>[8x]GIDPFTNTKWDYKNKENGPHRWDKLHKDFEVC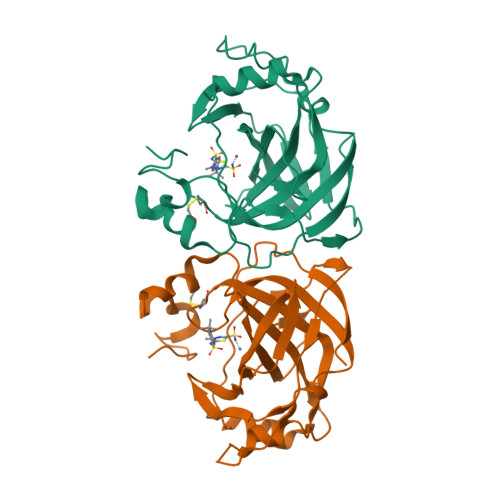KSGKSQSPINIEHYYHTQDKADLQFKYAASKPKAVFFTHHTLKASFEPTNHINYRGHDYVLDNVHFHAPMEFLINNKTRPLSAHFVHKDAKGRLLVLAIGFEEGKENPNLDPILEGIQKKQNFKEVALDAFLPKSINYYHFNGSLTAPPCTEGVAWFVIEEPLEVSAKQLAEIKKRMKNSPNQRPVQPDYNTVIIKSSAETR> SNMWVIGKSKAQDAKAIMVNGPQFGWYAPAYTYGIGLHGAGYDVTGNTPFAYPGLVFGHNGVISWGSTAGFGDDVDIFAERLSAEK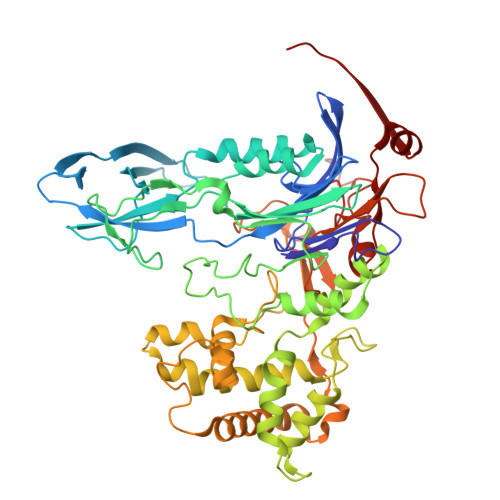PGYYLHNGKWVKMLSREETITVKNGQAETFTVWRTVHGNILQTDQTTQTAYAKSRAWDGKEVASLLAWTHQMKAKNWQEWTQQAAKQALTINWYYADVNGNIGYVHTGAYPDRQSGHDPRLPVPGTGKWDWKGLLPFEMNPKVYNPQSGYIANWNNSPQKDYPASDLFAFLWGGADRVTEIDRLLEQKPRLTADQAWDVIRQTSRQDLNLRLFLPTLQAATSGLTQSDPRRQLVETLTRWDGINLLNDDGKTWQQPGSAILNVWLTSMLKRTVVAAVPMPFDKWYSASGYETTQDGPTGSLNISVGAKILYEAVQGDKSPIPQAVDLFAGKPQQEVVLAALEDTWETLSKRYGNNVSNWKTPAMALTFRANNFFGVPQAAAEETRHQAEYQNRGTENDMIVFSPTTSDRPVLAWDVVAPGQSGFIAPDGTVDKHYEDQLKMYENFGRKSLWLTKQDVEAHKESQEVLHVQR9-{3-O-[(S)-thiophosphono]-alpha-L-lyxofuranosyl}-9H-purin-6-amine | C10 H14 N5 O6 P S | 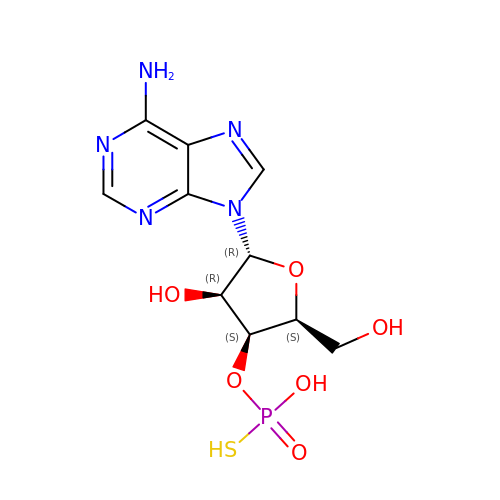GJFFFGIFPPIFQW-HGOUYRHRSA-N>GSDGGTLAMLRGLSEDTLEQLYALGFNQYQAGKWDDAQKIFQALCMLDHYDARYFLGLGACRQSLGLYEQALQSYSYGALMDINEPRFPFHAAECHLQLGDLDGAESGFYSARALAAAQPAHEALAARAGAMLEAV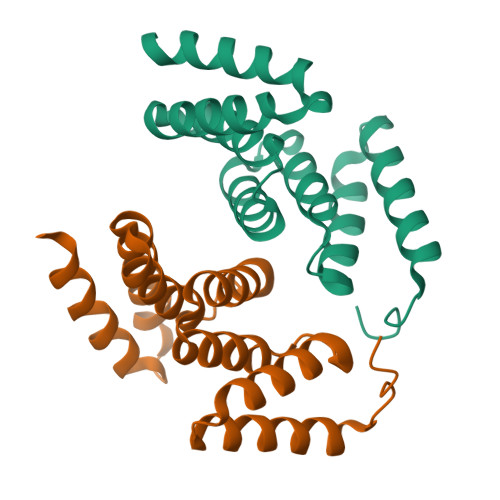TARKDR[2x]>[2x]MKITAVEPFILHLPLTSESISDSTHSITHWGVVGAKITTSDGIEGYGFTGTHAHLPSDRLITSCISDCYAPLLLGEDASDHSRLWTKLARYPSLQWVGRAGITHLALAAVDVALWDIKAKKAGVPLWHYLGGARTAGVEAYNTDIGWLSFTLEDLLAGSARAVEEDGFTRLKIKVGHDDPNIDIARLTAVRERVDSAVRIAIDGNGKWD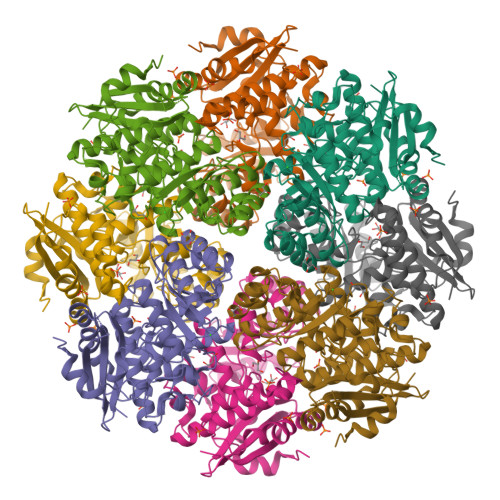LPTCQRFCAAAKDLDIYWFEEPLWYDDVTSHARLARNTSIPIALGEQLYTVDAFRSFIDAGAVAYVQPDVTRLGGITEYIQVADLALAHRLPVVPHAGEMSQVHVHLSYWHPASTILEYIPWIKDHFEEPIHVRDGVYKRPEQPGASTTPLAESFTRYGKAVK>[4x]GMSRGHCILAHGFESGPDALKVTALAEVAERLGWTHERPDFTDLDARRDLGQLGDVRGRLQRLLEIARAATE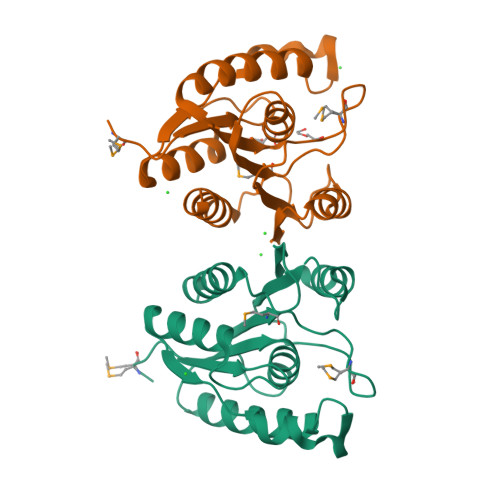KGPVVLAGSSLGSYIAAQVSLQVPTRALFLMVPPTKMGPLPALDAAAVPISIVHAWHDELIPAADVIAWAQARSARLLLVDDGHRLGAHVQAASRAFAELLQSL> MGHHHHHHGSSSCAVSGASGCLPPARSRIFKIIVIGDSNVGKTCLTYRFCAGRFPDRTEATIGVDFRERAVDIDGERIKIQLWDTAGQERFRKSMVQHYYRNVHAVVFVYDMTNMASFHSL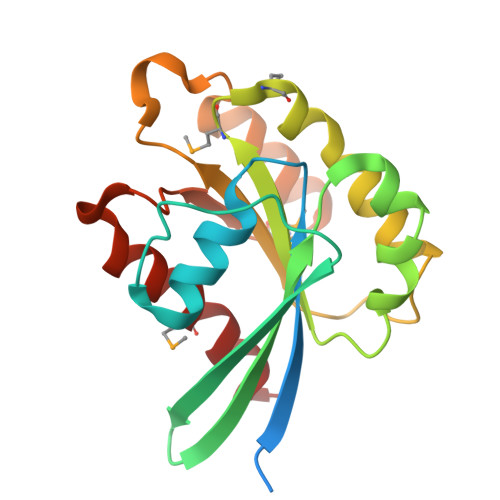PAWIEECKQHLLANDIPRILVGNKCDLRSAIQVPTDLAQKFADTHSMPLFETSAKNPNDNDHVEAIFMTLAHKLKSH methyl 2-[(2~{R})-1-(ethylcarbamoyl)-3-oxidanylidene-piperazin-2-yl]ethanoate 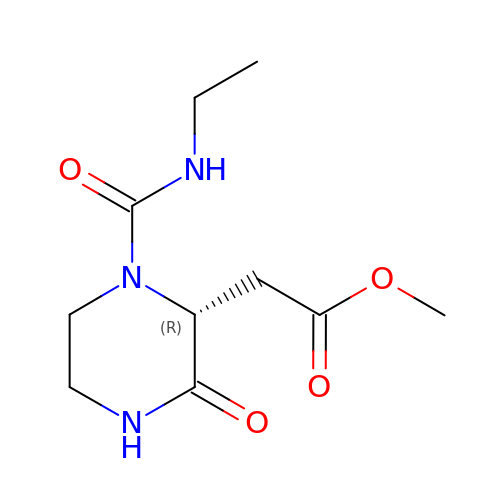| C10 H17 N3 O4 | RSMBLBWVWNZVOE-SSDOTTSWSA-N>[2x]GIDYDKLIVRFGSSKIDKELINRIERATGQRPHRFLRRGIFFSHRDMNQVLDAYENKKPFYLYTGRGPSSEAMHVGHLIPFIFTKWLQDVFNVPLVIQMTDDEKYLWKDLTLDQAYSYAVENAKDIIACGFDINKTFIFSDLDYMGMSSGFYKNVVKIQKHVTFNQVKGIFGFTDSDCIGKISFPAIQAAPSFSNSFPQ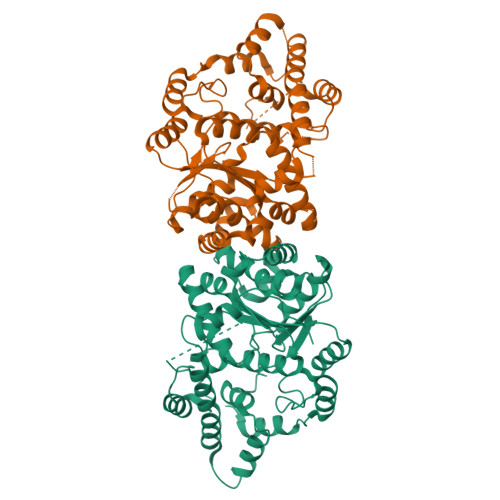IFRDRTDIQCLIPCAIDQDPYFRMTRDVAPRIGYPKPALLHSTFFPALQGAQTKMSASDPNSSIFLTDTAKQIKTKVNKHAFSGGRDTIEEHRQFGGNCDVDVSFMYLTFFLEDDDKLEQIRKDYTSGAMLTGELKKALIEVLQPLIAEHQARRKEVTDEIVKEFMTPRKLSFDFQKLAAALEHHHHHH2-[2-(3-chloro-4-methoxyphenyl)ethyl]-5-(3,5-dimethyl-1,2-oxazol-4-yl)-1-[(2S)-2-(morpholin-4-yl)propyl]-1H-benzimidazole | C28 H33 Cl N4 O3 | 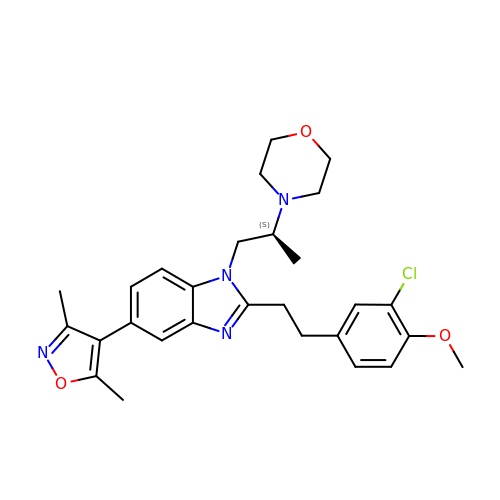GEPYBHCJBORHCE-SFHVURJKSA-N>[5x]HH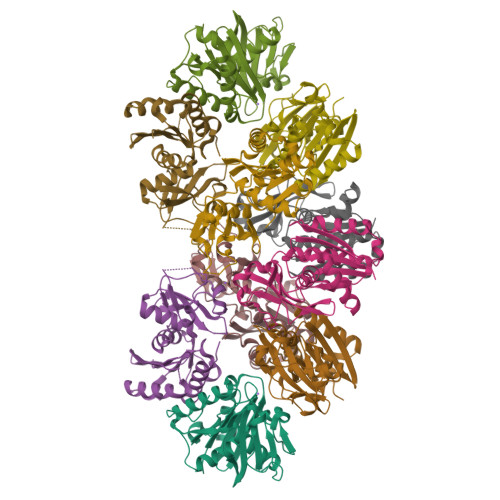HHHHMSTLLALDTSTEACSVALLHEGRALSHYEVIPRLHAQRLLPMVRDLLDEAGVALSAVDAIAFGRGPGAFTGVRIAIGVVQGLAFALQRPVLAVSDLAILAQRAYREQGAERVAAAIDARMDEVYWGCYQLQQGEMRLAGSEAVLPPERVAVPWDAAAADWFGAGTGWGYVERMPQRPVALDASLLPHAEDLLSLAGFAWARGEGVEAEQALPVYLRDNVATPKKAP>[2x]MHHHHHHRKAAGKYGNTLEFGHLVGGEEVLEGPLLERRNPSDREDVVARFPEADKDLVRKAALKAREAFAEWSRTPAPIRGQVLFNLVKILEREKPTLTRLMVREVGKTPKEAAGDVQEAIDTALFFASEGRRLYGQTVPSEMRDKELFTFRRPLGVVGIITAGNFPIAVPSWKLIPAVLTGNTVVWKPSEDAPTLSFVFAKLFEEAGLPPGVLNVVFGGGKGSTGQWMVELMDEGLFQKFAFTGSTQVGRWIGEVAGRNLIRPTLELGGKNPLVVMRDADLDLAVEGAWWSAFATGGQRCTSAGNILVDAPIYEEFKRRFLERVEATLVGNPLLHPEVTYGPFINERFFARWQEHYRVGEAEGARLLFGRGRITRENPYPRFLGDPEAGLYGWPTVWEVRPGTRLFTEEVFGPTINLVKVDGIEEAIAVANSTPYGLSSAIYTNHRHWAYLFKVGIRAGMTSINNATVGAEAHLPFGGVKASGNGGRESGIWVLEEYTYWHAVNEEYSGRLQLAQMDTGYVSPKAPTPWGEVLGL

Found in both prokaryotes and eukaryotes, aldehyde dehydrogenases (ALDH) (EC 1.2.1.3) constitute a large family of NAD(P)-dependent enzymes with molecular weights of 50–60 kDa. ALDHTt contains an unusually extended C-terminal arm forming novel interactions with the N-terminus in the quaternary structure which interacts closely with the substrate entry tunnel. The ALDHTt monomer is composed of the three domains common to all ALDHs: (i) The NAD(P)+ binding domain (1–125 + 148–261) comprising a Rossman fold, (ii) the catalytic domain (267–458) and (iii) the oligomerization domain (126–147 + 494–501). However, the presence in ALDHTt of an unusual extended arm that wrap the facing monomer through H-bonds and salt bridges shows for the first time how the tetramer is not merely a dimer-of-dimers carrying out their functions independent of each other, but that the interaction of the N- and C-termini in CS-related monomers may regulate active site access in NCS-related molecules.

The recombinant wild type crystals yielded a structure with a product molecule, propanoic acid, in monomer A and B. The product is ~6 Å from the catalytic thiol, which is in the attacking conformation, while the Glu261 can be observed in the “In” conformation in monomer B. Interestingly, the ligand, situated inside the aldehyde anchor loop within hydrogen bonding distance to Arg294, Thr296, Gly464 and Ala465, is observed in two different orientations. In monomer B, the carboxyl group of the propanoic acid is oriented toward the catalytic cysteine and is coordinated by hydrogen bonds with Arg294, Thr296 and Gly464. However, in monomer A the carboxyl group of the product is now oriented toward the aldehyde anchor loop and coordinated by the same residues as in monomer B in addition to Ala465 and Thr462 through a water-mediated hydrogen bond. Indeed, in the full-length recombinant protein Glu261 is observed in the “In” conformation, which may be indicative of an intermediate state depicting the molecule leaving the tunnel after catalysis, with repositioning of the glutamic acid. The different orientations of the product in monomers A and B is likely to provide snapshots of product handling throughout the aldehyde anchor loop. It is worthy to note that a similar product orientation was previously observed with ALDH1A336.> MSIIEMRDVVKKYDNGTTALRGVSVSVQPGEFAYIVGPSGAGKSTFIRSLYREVKIDKGSLSVAGFNLVKIKKKDVPLLRRSVGVVFQDYKLLPKKTVYENIAYAMEVIGENRRNIKRRVMEVLDLVGLKHKVRSFPNELSGGEQQRIAIARAIVN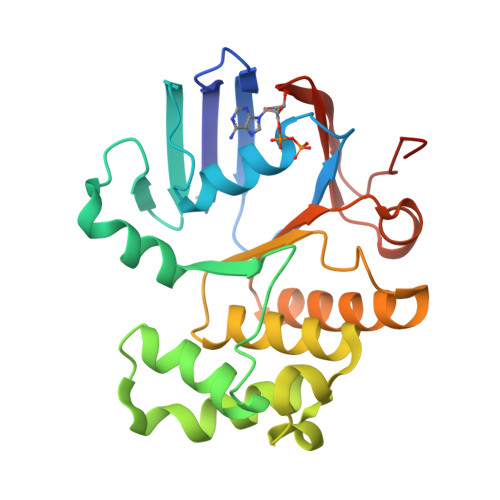NPKVLIADEPTGNLDPDNSWEIMNLLERINLQGTTILMATHNSQIVNTLRHRVIAIENGRVVRDESKGEYGYDD> GPLGSKKRQCKVLFEYIPQNEDELELKVGDIIDINEEVEEGWWSGTLNNKLGLFPSNFVKELEVT;> RPTPRPVPMKRH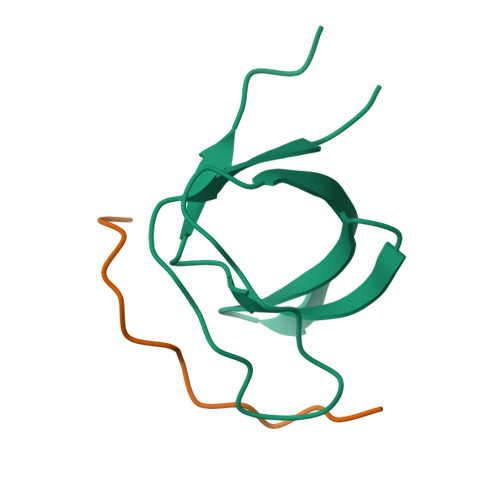IFRS> GAGCAGCCTGTXTGGACAT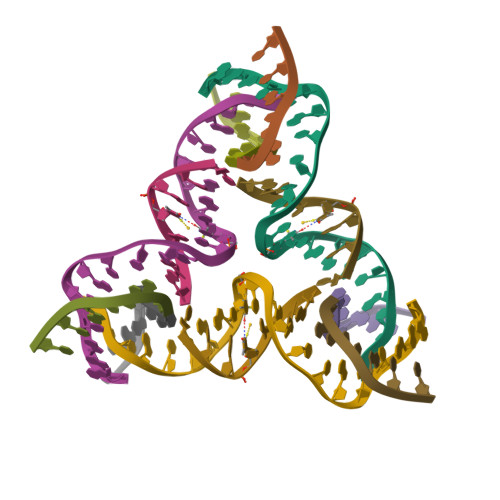CA;> CCAXACA;> GGCTGCT;> CTGATGT> GAMSETSVNRGPEKIRPECFELLRVLGKGGYGKVFQVRKVTGANTGKIFAMKVLKKAMIVRNAKDTAHTKAERNILEEVKHPFIVDLIYAFQTGGKLYLILEYLSGGELFMQLEREGIFMEDTACFYLA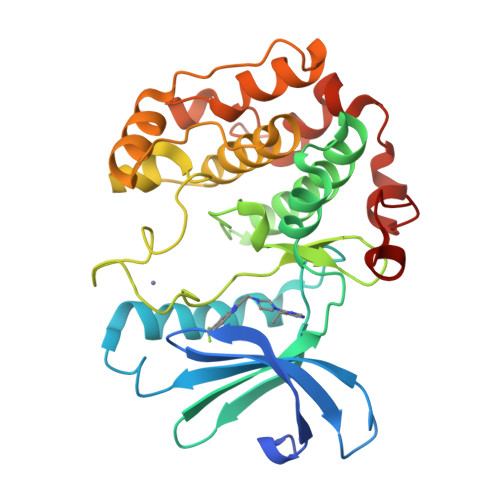EISMALGHLHQKGIIYRDLKPENIMLNHQGHVKLTDFGLCKESIHDGTVTHTFCGTIEYMAPEILMRSGHNRAVDWWSLGALMYDMLTGAPPFTGENRKKTIDKILKCKLNLPPYLTQEARDLLKKLLKRNAASRLGAGPGDAGEVQAHPFFRHINWEELLARKVEPPFKPLLQS>[4x]XGSIGAASMEFCFDVFKELKVHHANENIFYCPIAIMSALAMVY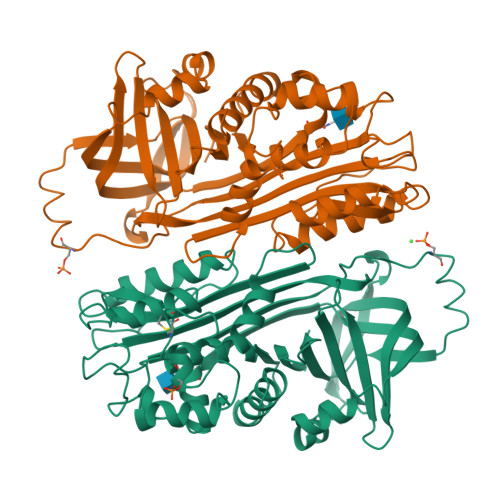LGAKDSTRTQINKVVRFDKLPGFGDSIEAQCGTSVNVHSSLRDILNQITKPNDVYSFSLASRLYAEERYPILPEYLQCVKELYRGGLEPINFQTAADQARELINSWVESQTNGIIRNVLQPSSVDSQTAMVLVNAIVFKGLWEKAFKDEDTQAMPFRVTEQESKPVQMMYQIGLFRVASMASEKMKILELPFASGTMSMLVLLPDEVSGLEQLESIINFEKLTEWTSSNVMEERKIKVYLPRMKMEEKYNLTSVLMAMGITDVFSSSANLSGISSAESLKISQAVHAAHAEINEAGREVVGSAEAGVDAASVSEEFRADHPFLFCIKHIATNAVLFFGRCVSP> QQAGTNTAENHPQLQSQQCTTSGGCKPLSTKVVLDSNWRWVHSTSGYTNCYTGNEWDTSLCPDGKTCAANCALDGADYSGTYGITSTGTALTLKFVTGSNVGSRVYLMADDTHYQLLKLLNQEFTFDVDMSNLPCGLNGALYLSAMDADGGMSKYPGNKAGAKYGTGYCDSQCPKDIKFINGEANVGNWTETGSNTGTGSYGTCCSEMDIWEANNDAAAFTPHPCTTTGQTRCSGDDCARNTGLCDGDGCDFNSFRMGDKTFLGKGMTVDTSKPFTVVTQFLTNDNT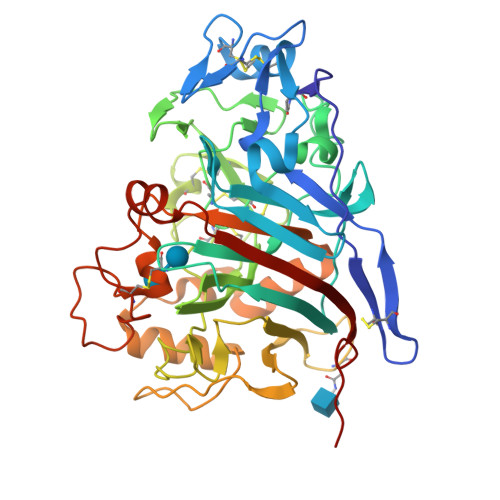STGTLSEIRRIYIQNGKVIQNSVANIPGVDPVNSITDNFCAQQKTAFGDTNWFAQKGGLKQMGEALGNGMVLALSIWDDHAANMLWLDSDYPTDKDPSAPGVARGTCATTSGVPSDVESQVPNSQVVFSNIKFGDIGSTFSGTS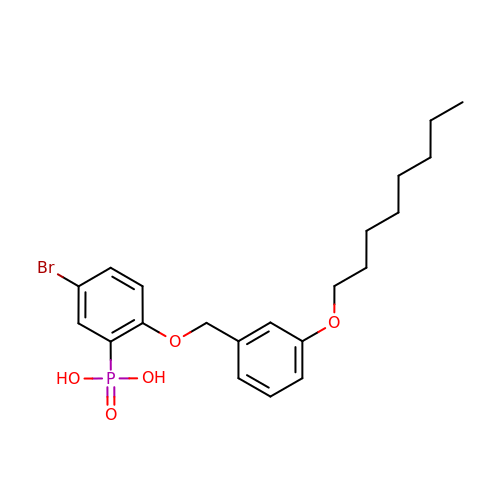(5-bromo-2-{[3-(octyloxy)benzyl]oxy}phenyl)phosphonic acid | C21 H28 Br O5 P | XTZIHTNEICPHNT-UHFFFAOYSA-N Here, we identify archaeal proteins that are homologs of fusexins, a superfamily of fusogens that mediate eukaryotic gamete and somatic cell fusion, as well as virus entry. The crystal structures of HAP2/GCS1 from Chlamydomonas and Arabidopsis showed remarkable structural conservation without sequence similarity. This superfamily of fusion proteins was named fusexins: fusion proteins essential for sexual reproduction and exoplasmic merger of plasma membranes. The crystal structure of a trimeric archaeal fusexin (Fusexin1 or Fsx1) reveals an archetypical fusexin architecture with unique features such as a six-helix bundle and an additional globular domain. Ectopically expressed Fusexin1 can fuse mammalian cells, and this process involves the additional globular domain and a conserved fusion loop.

Fsx1E is a monomer in solution but crystallized as a homotrimer in the presence of 2.5 M NaCl, 0.2 M CaCl2. However, we could determine the structure of Fsx1E at 2.3 Å resolution by running MR with a combination of fragments from ab initio predictions generated by AlphaFold229. Each protomer consists of four domains, the first three of which match the approximate dimensions and relative arrangement of domains I–III of known fusexins in their post-fusion conformation; accordingly, fold and interface similarity searches identify HAP2 as the closest structural homolog of Fsx1E, followed by viral fusexins and C. elegans EFF-1. Fsx1 domains I and III are relatively sequence-conserved among archaeal homologs and closely resemble the corresponding domains of HAP2 (RMSD 2.1 Å over 218 Cα), including the invariant disulfide bond between domain III strands βC and βF23 (C3389–C4432). On the other hand, Fsx1 domain II shares the same topology as that of HAP2 but differs significantly in its secondary structure elements and their relative orientation, as well as disulfide bonds. In particular, Fsx1 domain II is characterized by a four-helix hairpin, whose N-terminal half interacts with the same region of the other two subunits to generate a six-helix bundle around the molecule’s three-fold axis. Notably, unlike previously characterized viral and eukaryotic fusexins, Fsx1 also contains a fourth globular domain conserved among archaeal homologs. In addition to being coaxially stacked with domain III as a result of a loop/loop interaction stabilized by the C5457–C6477 disulfide, domain IV contributes to the quaternary structure of the protein by interacting with domain II of the adjacent subunit to which domain III also binds. The Fsx1E monomer has a net charge of −67, and another feature stabilizing its homotrimeric assembly is a set of Ca2+ and Na+ ions that interacts with negatively charged residues at the interface between subunits.

>[3x]ETGDSITYNSGTSEFFDGDVFAIEVTADQSTDEIDIYLGASELSEKTDGEVNQDLSIEFTHQDSKLKYSTSTSDELRDIVTLTTYYEDGFDTEQDAIDAIKSDCYDLNQNGNGSGRYSRYYSVTSPVYDYEIYCFQKNEKLATPAYIDNPDEIFTAKAELQAGDKTIQSATLSNGDAGDGTVTDLGDSKISWNGNLDLGASEPENSRVIALYSNDFENGWRIGNKQSYEDYKTFIGGGDAYDLLIDWQDGTYTASEVEDELVNTDANQAVEEASSSTTDLVNAKVKDSSLDTGSFVYDTPELLSYPSFTVYVDAGENGYIEVTKPTGDPDIISTSSTEIKEGDEGTVCATVENVGDGEGEFSGRLSSCGEGFSIVDDQNTKNVGAGESVTYSFDVAFSSVSSESKEISGSCTFEVNGVESSDSTSVSVTGIQQSECNPGDQRREKNENDRWEIYTCQDNGLTYEYDVTCAEDEKAVAQGDNQFSCEKQDDDSGGGDNTGSDSGLFSNLFGGSGSLEHHHHHHHH> MKRVFLLYIIGILLTLFLPLIQTQSAVSLPPLYVEDAVNAEIQQLWSKSPTGVYAFHEAPSVNNSFWPDDNAKFLESIAPWWQSYSSYVNSTLQFLQQSDVNGLFIKRFEYPLNPLQSITIGNLSGYTNGFYDIVGNPLLNSMRIATYYNPTLAVTYLFGNVVQYPNGILVNIEQGLENPITDGGFGGTGGQNPPWESLNSSSLVNDSIVSIVNNAKTYLNLTGPTFFGTPSEELQYNFPIVNVLPHYLAFQNVNGILGQYNYQGKFIPFNVTLVLQSSSINRIYLEFIWENSTSGTYVLTDIPVYFT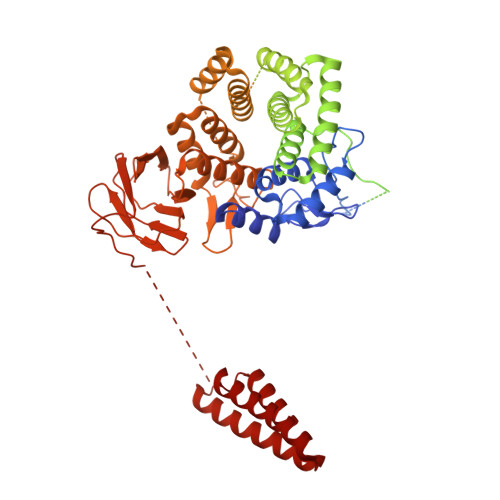ANGQWQQVVVTVPASAWPKYWNLGALSAVPLLIGIGLDLPGSSPSQTGPTGVYVGDIATNYPTTFGPQFNVTNKGSYVVFNESWKSDSLGATFWIAYVLGQGNAIEVLASAPVNQSWIYVGYNGLATIGTGYTILETPSGILKNYQNSGNISWTYLGPNFGKWMLLSTNYAPNWIGDFQMLFIFPMAGTSNPYMDTLNNAVYMGDPTEVRNTLYFGNYTTLPGYFQWVQIAYQNDGNTSGVFGFFLIPSVDYLVNPSVIVNDMFPSSLTAYSPSSIPNYWWEAVWGENYYEGEIIYALALLGKYGNSQALQMAQQAWLSYYNQLKAYNGATYTSSLARFIMATILLYNITGNTQYSNAYTQLANWLLQYQNQSKYAYVYIPMWYHKDVDVPSVNGFATYGYIINRTAQMDVGTVISGTSIGLNFFEDIPLNTSYGIYLLTNGTGKLPFTYQNVLNVSGTFITYLYMNGGGTATTANITITVQIAYNGNVLQTIGTAAVDNVPIQPGGISGSPPFYPVKIVVPVLTTVNAPPGSTLIIGWNIKAPQTVYVLIDSTNGPSNVTIPLSWPNPFYGLFTIPKIYNPNPGVHNYPQPYFLDISAMAGQAMMALYAVTKNITYLLDAQLVMNAIHYGPVPMPTYGILGVPNPPVEPRLWVYANYSTVDADYYTYKSELVSEFGDAIGNNTLASLAISRVWQRTSYTYPTSYIYYVARYGSGLQMNSETQPWGDVATQFYVNTWSPSNLDLFWASLPNNNYITNQTWNGTALFIHLYAYQQSQVQLIFLTTTVNFNVLVNGNYTNYEANHQIMQIAPTLEPGPNTIIIIPNPKNQVSQNTNISTTTTTSPLSNAISGLGITLTQNELMLLGFVIYFVIIMVTYGVSRNKTITVLSSIVAVAIVYALALWPTYMAFILGAVGFFMLFYSISRREEE> MSKPQPIAAANWKCNGSQQSLSELIDLFNSTSINHDVQCVVASTFVHLAMTKERLSHPKFVIAAQNAIAKSGAFTGEVSLPILKDFGVNWIVLGHSERRAYYGETNEIVADKVAAAVASGFMVIACIGETLQERESGRTAVVVLTQIAAIAKKLKKADWAKVVIAYEPVWAIGTGKVLTPQQAQEAHALIRSWVSSKIGADVAGELRILYG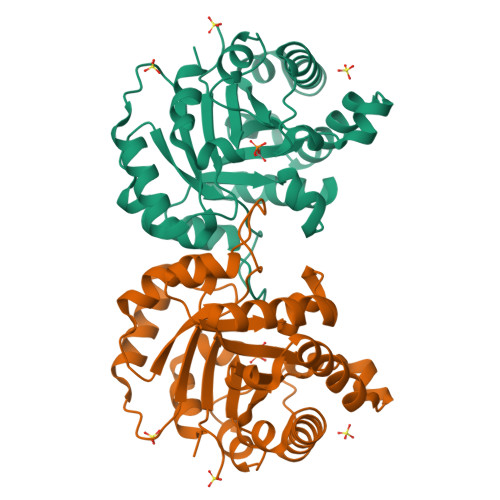GSVNGKNARTLYQQRDVNGFLVGGASLKPEFVDIIKATQ>KNKVNRSFVDLGISTQRKIVYELYFAVKYLSKNKVGAIITLQRNILLDSLRTDGVKIDSLINSSLLIAIFQKSSPLHDGAVIIVDDRILYASTYFSVSESTLEDRYGARHRAALGISEVSDSITVVVSEQSGEVVIVRDANFFKVTNLETFTEVLTKELNSSQTNTAKKHHH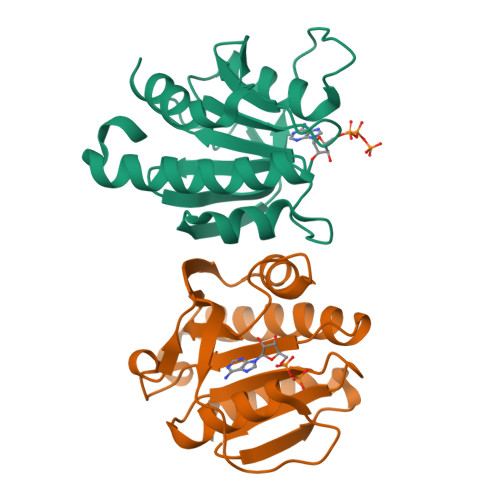HHH[2x]> PKQLRFEGERVTWIQASTLKELLDLKAQHPEAKLVVGNTEIGIEMKFKNQLFPMIICPAWIPELNAVEHGPEGISFGAACALSSVEKTLLEAVAKLPTQKTEVFRGVLEQLRWFA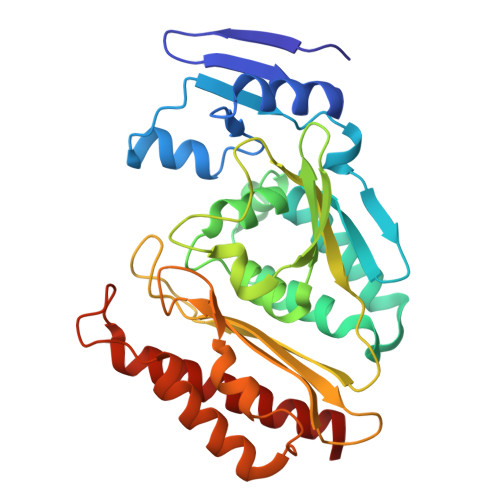GKQVKSVASLGGNIITASPISDLNPVFMASGTKLTIVSRGTRRTVPMDHTFFPSYRKTLLGPEEILLSIEIPYSREDEFFSAFKQASRREDDIAKVTCGMRVLFQPGSMQVKELALCYGGMADRTISALKTTQKQLSKFWNEKLLQDVCAGLAEELSLSPDAPGGMIEFRRTLTLSFFFKFYLTVLKKLG>[4x]GHMSPEREITLVNLKKDAKYG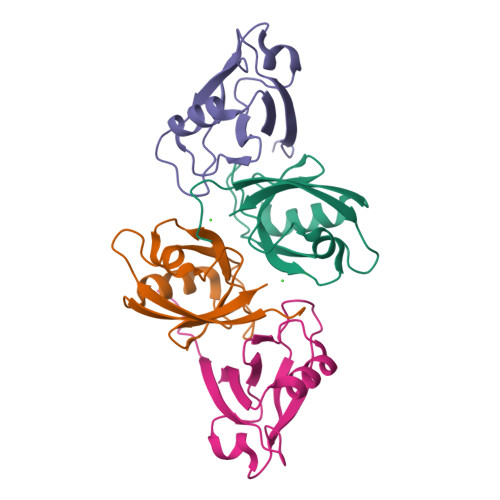LGFQIIGGEKMGRLDLGIFISSVAPGGPADLDGCLKPGDRLISVNSVSLEGVSHHAAIEILQNAPEDVTLVISQP>[4x]GMSFDINWSTLESDNRLNDLIRKHLNSYLQNTQLPSYVSNLRVLDFDLGKVGPAITLKEITDPLDEFYDSIREEADQETEENNDNKEDSEHICPDRTIANHEGPKDDFEAPVVMPSPNDIQFLLEVEYKGD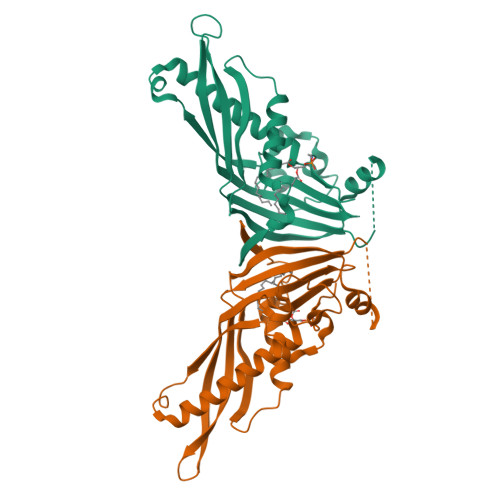LLVTIGADLVLNYPVEKFMTLPVKLSISDIGLHSLCIVACLSKQLFLSFLCDVSDPALDDNQTVLDPKGPILAATKPLERISIVRSMKIETEIGEQYQGQGSVLRSVGELEQFLFTIFKDFLRKELAWPSWINLDFNDGDE>DYKDDDDKDYKDDDDKDYKDDDDKHHHHHHENLYFQGVSRMGWGGRRRRLGRWGDLGPGSVPLLPMPLPPPPPPSCRGPGGGRISIFSLSPAPHTRSSPSSFSPPTAGPPCSVLQGTGASQSCHSALPIPATPPTQAQPAMTPASASPSWGSHSTPPLAPATPTPSQQCPQDSPGLRVGPLIPEQDYERLEDCDPEGSQDSPIHGEEQQPLLHVPEGLRGSWHHIQNLDSFFTKIYSYHQRNGFACILLEDVFQLGQFIFIVTFTTFLLRCVDYNVLFANQPSNHTRPGPFHSKVTLSDAILPSAQCAERIRSSPLLVLLLVLAAGFWLVQLLRSVCNLFSYWDIQVFYREALHIPPEELSSVPWAEVQSRLLALQRSGGLCVQPRPLTELDIHHRILRYTNYQVALANKGLLPARCPLPWGGSAAFLSRGLALNVDLLLFRGPFSLFRGGWELPHAYKRSDQRGALAARWGRTVLLLAALNLALSPLVLAWQVLHVFYSHVELLRREPGALGARGWSRLARLQLRHFNELPHELRARLARAYRPAAAFLRTAAPPAPLRTLLARQLVFFAGALFAALLVLTVYDEDVLAVEHVLTAMTALGVTATVARSFIPEEQCQGRAPQLLLQTALAHMHYLPEEPGPGGRDRAYRQMAQLLQYRAVSLLEELLSPLLTPLFLLFWFRPRALEIIDFFHHFTVDVAGVGDICSFALMDVKRHGHPQWLSAGQTEASLSQRAEDGKTELSLMRFSLAHPLWRPPGHSSKFLGHLWGRVQQDAAAWGATSARGPS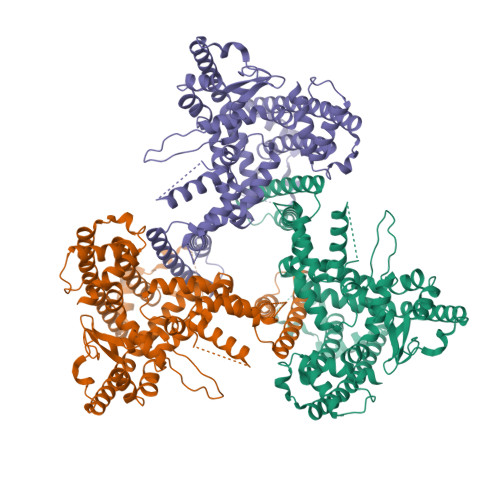TPGVLSNCTSPLPEAFLANLFVHPLLPPRDLSPTAPCPAAATASLLASISRIAQDPSSVSPGGTGGQKLAQLPELASAEMSLHVIYLHQLHQQQQQQEPWGEAAASILSRPCSSPSQPPSPDEEKPSWSSDGSSPASSPRQQWGTQKARNLFPGGFQVTTDTQKEPDRASCTD[3x]>[2x]SQVKSKA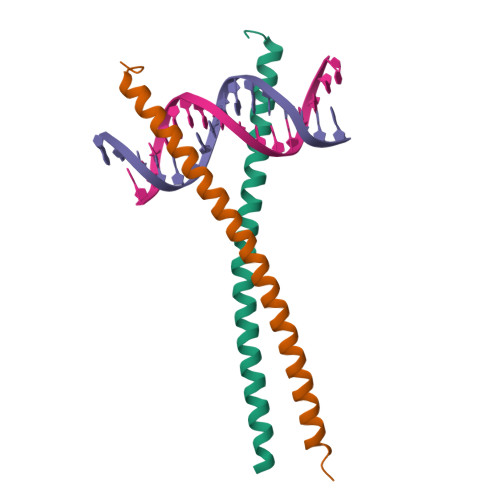KKTVDKHSDEYKIRRERNNIAVRKSRDKAKMRNLETQHKVLELTAENERLQKKVEQLSRELSTLRNLFKQLPE> MHMKNIKKNQVMNLGPNSKLLKEYKSQLIELNIEQFEAGIGLILGDAYIRSRDEGKTYCMQFEWKNKAYMDHVCLLYDQWVLSPPHKKERVNHLGNLVITWGAQTFKHQAFNKLANLFIVNNKKTIPNNLVENYLTPMSLAYWFMDDGGKWD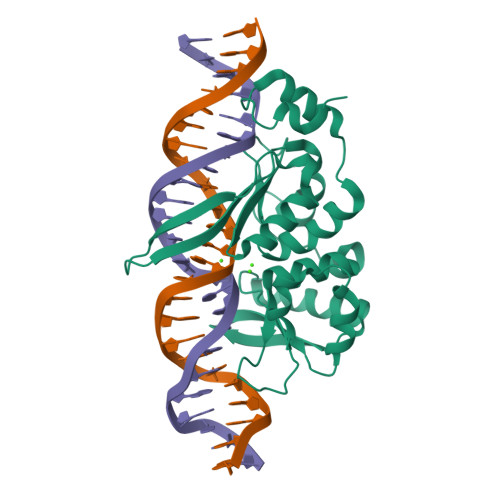YNKNSTNKSIVLNTQSFTFEEVEYLVKGLRNKFQLNCYVKINKNKPIIYIDSMSYLIFYNLIKPYLIPQMMYKLPNTISSETFLK>[2x]ETGGSWAQVKLLESGGKVTHEGQSVTLTCKASGFNFKDYDMSWHWSPSGSNRQLVASISSKTGSKTEYKPRIQGRAYITRNNEANTVSLTLIQLRKEDSGIYYCAKLENVGGLSRYIIREQWGNFGPGTKLTVLPLEKTLLTESGGGTYQAGKTLSLKCQTSGFQFKTSQLDWYLWTPGHAPLWLTGLNSSSTDATEGRITSSREDNKNQIFLQIEDLGLRDSGQYHCARRVGNGDDTDKLVFGLGTRVIVEPRPQAPLSPSVFLVRDQNAVACLIRNFYPKELHVSLTSSGTLIS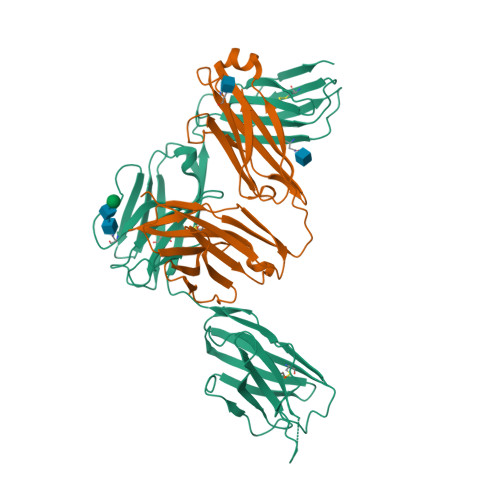AQNLTLAPMATGTYSAIHIGRVGENDAITCSVKHLEKEIHMSHQAGSLVPR;>ETGVALEQRPISITRNAKQSASLNCKILNPVSDYVHWYRSQEGRAPERLLVYSRSKSESVPDPGFSADKVRAYKGADDTCRLIVSDLQVSDSGVYHCASWDGRVKVFGEGTRLIVTESAFKKKPPKPIFFLPTSEEIKQKQSGTYICLLEDFFPNVVKTYWKEDGNSQPLDAQFGPITGGGNSYSQVSWLTVKEDVLRKNLTYFYQHEDLGMEPKAFSISSVREKGSLVPR[2x]>MAEIKHYQFNVVMTCSGCSGAVNKVLTKLEPDVSKIDISLEKQLVDVYTTLPYDFILEKIKKTGKEVR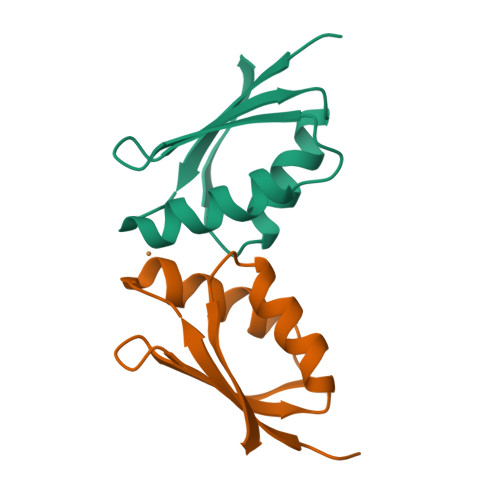SGKQL[8x]> GSDEDFVTCYSVLKFINANDGSRLHSHDVKYGSGSGQQSVTAVKNSDDINSHWQIFPALNAKCNRGDAIKCGDKIRLKHLTTGTFLHSHHFTAPLSKQHQEVSAFGSEAESDTGDDWTVICNGDEWLESEQFKLRHAVTGSYLSLSGQQFGRPIHGQREVVGTDSITGGSAWKVAEG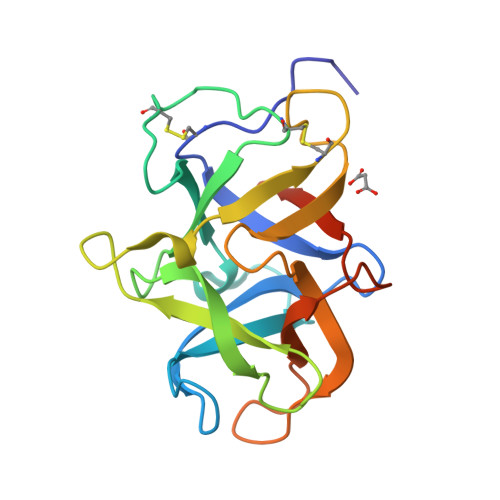IYIKHQQKDL>UAGCUCC[2x];>[2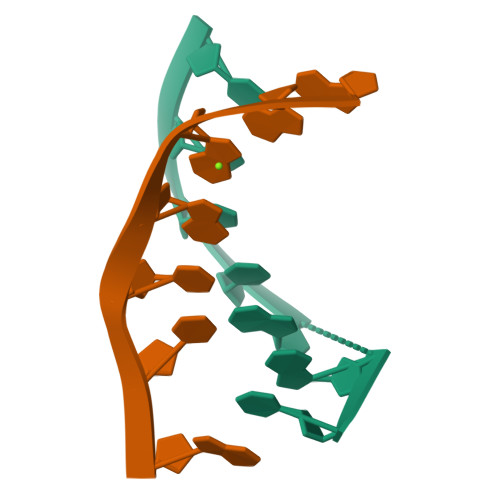x]GGAGCTA> AVTNEEVNQMIEDRKVDFNQNWYFKLNANSKEAIKPDADVSTWKKLDLPYDWSIFNDFDHESPAQNEGGQLNGGEAWYRKTFKLDEKDLKKNVRLTFDGVYMDSQVYVNGQLVGHYPNGYNQFSYDITKYLQKDGRENVIAVHAVNKQPSSRWYSGSGIYRDVTLQVTDKVHVEKNGTTILTPKLEEQQHGKVETHVTSKIVNTDDKDHELVAEYQIVERGGHAVTGLVRTASRTLKAHESTSLDAILEVERPKLWTVLNDKPALYELITRVYRDGQLVDAKKDLFGYRYYHWTPNEGFSLNGERIKFHGVSLHHDHGALGAEENYKAEYRRLKQMKEMGVNSIRTTHNPASEQTLQIAAELGLLVQEEAFDTWYGGKKPYDYGRFFEKDATHPEARKGEKWSDFDLRTMVERGKNNPAIFMWSIGNEIGEANGDAHSLATV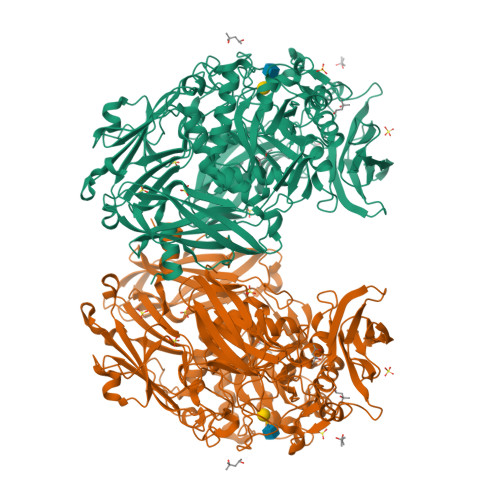KRLVKVIKDVDKTRYVTMGADKFRFGNGSGGHEKIADELDAVGFNYSEDNYKALRAKHPKWLIYGSQTSSATRTRGSYYRPERELKHSNGPERNYEQSDYGNDRVGWGKTATASWTFDRDNAGYAGQFIWTGTDYIGEPTPWHNQNQTPVKSSYFGIVDTAGIPKHDFYLYQSQWVSVKKKPMVHLLPHWNWENKELASKVADSEGKIPVRAYSNASSVELFLNGKSLGLKTFNKKQTSDGRTYQEGANANELYLEWKVAYQPGTLEAIARDESGKEIARDKITTAGKPAAVRLIKEDHAIAADGKDLTYIYYEIVDSQGNVVPTANNLVRFQLHGQGQLVGVDNGEQASRERYKAQADGSWIRKAFNGKGVAIVKSTEQAGKFTLTAHSDLLKSNQVTVFTGKKEG Ras suppressor protein 1 (Rsu1), a leucine-rich repeat (LRR)-containing protein conserved from human to worms, was recognized as a major FA component and is important for FA formation and cell motility. Among the IAC components, tripartite integrin-linked kinase (ILK) associates with another two key players PINCH and Parvin to form the ILK/PINCH/Parvin (IPP) complex, which acts as an essential platform to recruit many proteins for the FA formation and signaling and provide a linkage between FA and actin cytoskeleton. Here, we solved the crystal structures of the Rsu1/PINCH1 complex and found that Rsu1 strongly binds to PINCH1 through a large concave surface on its LRR solenoid. The cellular data supported the inhibitory effect of Rsu1 on the IPP complex. These results indicated that Rsu1, by interacting with PINCH1 and preventing PINCH1 from binding to actin, modulates actin dynamics at the FA and thereby regulates the stress fiber formation and cell adhesion dynamics.

We prepared the Rsu1/PINCH1 complex by combinatorial usage of the purified fragments that contains the elements necessary and sufficient for the Rsu1/PINCH1 interaction and successfully obtained the crystals of the Rsu1ΔC/PINCH1_LIM5C and Rsu1/PINCH1_LIM45C complexes. The complex structures of Rsu1ΔC/PINCH1_LIM5C with one crystal form at 1.65 Å resolution and Rsu1/PINCH1_LIM45C with two different crystal forms at 2.2 Å and 3.15 Å resolution respectively were determined by the molecular replacement method. In the Rsu1/PINCH1_LIM45C complex, the nine LRRs of Rsu1 form a curved solenoid capped by the helical regions in the both N- and C-termini, named N-cap and C-cap, respectively. The N-cap consists of the α1-helix while the C-cap contains three α-helices (α2–4). Both the two helical regions cap the LRR-solenoid by forming extensive hydrophobic interactions with LRR1–2 and LRR8–9, respectively. All the nine LRRs adopt the typical LRR-folding by using conserved leucine residues to form the hydrophobic core except for a few short loops inserted in LRR1, 5, and 9. Consistent with our biochemical finding, the LRR-solenoid of Rsu1 interacts with both the LIM5 domain and the C-terminal tail (C-tail, folded as a α-helix) of PINCH1 through the concave surface of the solenoid, mainly formed by the parallel β-sheet and the flanking loop regions. However, the LIM4 domain in PINCH1 adopts different orientations as observed in the two crystal forms of the Rsu1/PINCH1_LIM45C complex, indicating the intrinsic, structural flexibility between the LIM4 and LIM5 domains. Interestingly, although separately distributed at the interface, the polar interactions are well organized together by forming a hydrogen-bond network. In this network, two buried water molecules, conserved in both the Rsu1ΔC/PINCH1_LIM5C and Rsu1/PINCH1_LIM45C complex structures, critically coordinate three clusters of the polar interactions as highlighted in Figure 3D.

>GAMGSMSKSLKKLVEESREKNQPEVDMSDRGISNMLDVNGLFTLSHITQLVLSHNKLTMVPPNIAELKNLEVLNFFNNQIEELPTQISSLQKLKHLNLGMNRLNTLPRGFGSLPALEVLDLTYNNLSENSLPGNFFYLTTLRALYLSDNDFEILPPDIGKLTKLQILSLRDNDLISLPKEIGELTQLKELHIQGNRLTVLPPELGNLDLTGQKQVFKAENNPWVTPIADQFQLGVSHVFEYIRSETYKYLYGRHMQANPEPPKKNNDKSKKISRKPLAAKNR[2x];>GPGSMGVPICGACRRPIEGRVVNAMGKQWHVEHFVCAKCEKPFLGHRHYERKGLAYCETHYNQLFGDVCFHCNRVIEGDVVSALNKAWCVNCFACSTCNTKLTLKNKFVEFDMKPVCKKCYEKFPLELKKRLKKLAETLGRK[2x]>[2x]GPRMAFTNYSSLNRAQLTFEYLHTNSTTHEFLFGALAELVDNARDADATRIDIYAERREDLRGGFMLCFLDDGAGMDPSDAASVIQFGKSAKRTPESTQIGQYGNGLKSGSMRIGKDFILFTKKEDTMTCLFLSRTFHEEEGIDEVIVPLPTWNARTREPVTDNVEKFAIETELIYKYSPFRTEEEVMTQFMKIPGDSGTLVIIFNLKLMDNGEPELDIISNPR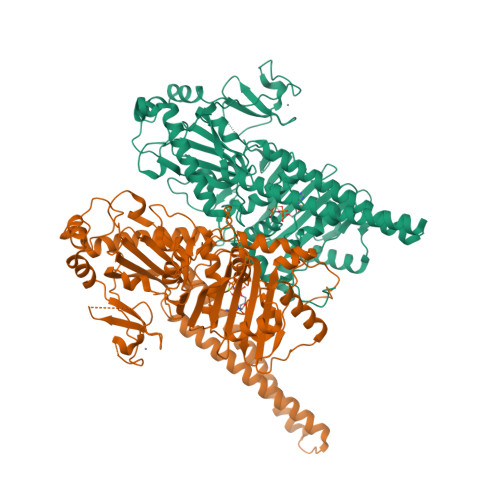DIQMAETSPEGTKPERRSFRAYAAVLYIDPRMRIFIHGHKVQTKRLSCCLYKPRMYKYTSSRFKTRAEQEVKKAEHVARIAEEKAREAESKARTLEVRLGGDLTRDSRVMLRQVQNRAITLRREADVKKRIKEAKQRALKEPKELNFVFGVNIEHRDLDGMFIYNCSRLIKMYEKVGPQLEGGMACGGVVGVVDVPYLVLEPTHNKQDFADAKEYRHLLRAMGEHLAQYWKDIAIAQRGIIKFWDEFGYLSANWNQPPSSELRYKRRRAMEIPTTIQCDLCLKWRTLPFQLSSVEKDYPDTWVCSMNPDPEQDRCEASEQKQKVPLGTFRKDMKTQEEKQKQLTEKIRQQQEKLEALQKTTPIRSQADLKKLPLEVTTRPST>GSTIQEVREGLPIEKMADFSLEELLGMAIKAEIGAREFYKSLAEKIKIEALKEKINWLAEEEKKHEALLRKLYSQMFPGKEVVFPK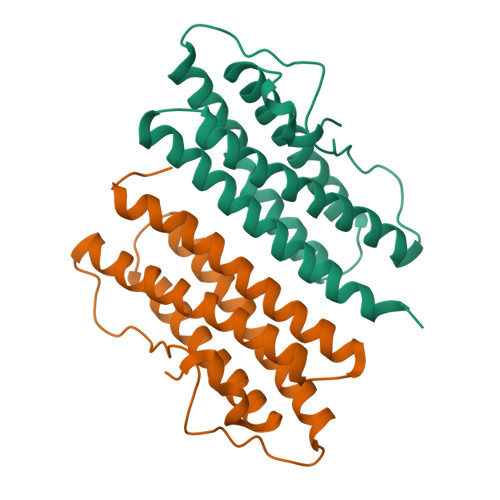EHIGPELQPVARELEKVQDIIDLIRWAMKAEEIAAEFYLKLEEMVKEEEKKRLMRYLADMERGHYYTLRAEYELLLNWEMYSQMMHIGP[2x]> MSLDSPLYGRSFADDKMRELFSAQSFISRCVETEVALARAQARLGIIPEDAAAGITAAARTFAPEMERLRDDTEIVGYPILPLVEQLSAHAGEAGKYLHWGATTQDIMDTATVLQIRDGLALISRRIESVRKALAALARNHRDTPMAGRTHLQHALPVTFGYKAA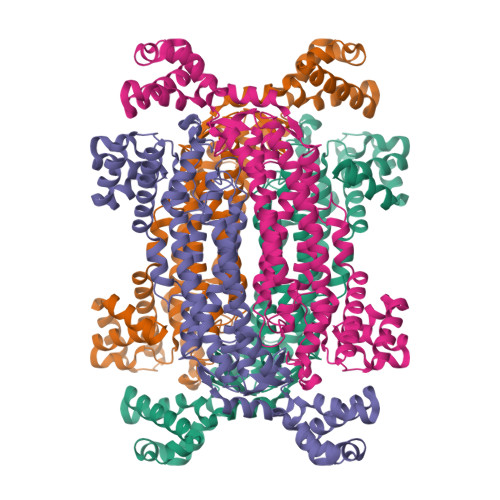VWLSAFDRHAARLEEISPRVLVVEFSGASGTLASLGTRGLDVQRELARELNLGVPSITWHSARDAVAETVQFLALVSGSLGKLAMDISIMMTTELGEVAEPFVRHRGASSTMPQKQNPVSCELILAGARIVRNHATSMLDAMIHDFERATGPWHLEWSAVPEGFAVASGILYQAEFMLGGLQVFPDRMRENLDHSRGLIVAEAVMMALAPHTGRKEAHDIVYLGCRRAVEDKTGLFEVLRTMPEVAKPLGEEALRDLTDPRNYLGSAGAMVDNVLGGREGHHHHHH> MVKLAEFSRTATFAWSHDKIPLLVSGTVSGTVDANFSTDSSLELWSLLAADSEKPIASLQVDSKFNDLDWSHNNKIIAGALDNGSLELYSTNEANNAINSMARFSNHSSSVKTVKFNAKQDNVLASGGNNGEIFIWDMNKCTESPSNYTPLTPGQSMSSVDEVISLAWNQSLAHVFASAGSSNFASIWDLKAKKEVIHLSYTSPNSGIKQQLSVVEWHPKNSTRVATATGSDNDPSILIWDLRNANTPLQTLNQGHQKGILSLDWCHQDEHLLLSSGRDNTVLLWNPESAEQLSQFPARGNWCFKTKFAPEAPDLFACASFDNKIEVQTLQNLTNTLDEQETETKQQESETDFWNNVSREESKEKPSVFHLQAPTWYGEPSPAAHWAFGGKLVQITPDGKGVSITNPKISGLESNTTLSEALKTKDFKPLINQRLVKVIDDVNEEDWNLLEKLSMDGTEEFLKEALAFDNDESDAQDDANNEKEDDGEEFFQQIETNFQPEGDFSLSGNIEQTISKNLVSGNIKSAVKNSLENDLLMEAMVIALDSNNERLKESVKNAYFAKYGSKSSLSRILYSISKREVDDLVENLDVSQWKFISKAIQNLYPNDIAQRNEMLIKLGDRLKENGHRQDSLTLYLAAGSLDKVASIWLSEFPDLEDKLKKDNKTIYEAHSECLTEFIERFTVFSNFINGSSTINNEQLIAKFLEFINLTTSTGNFELATEFLNSLPSDNEEVKTEKARVLIASGKSLPAQNPATATTSKAKYTNAKTNKNVPVLPTPGMPSTTSIPSMQAPFYGMTPGASANALPPKPYVPATTTSAPVHTEGKYAPPSQPSMASPFVNKTNSSTRLNSFAPPPNPYATATVPATNVSTTSIPQNTFAPIQPGMPIMGDYNAQSSSIPSQPPINAVSGQTPHLNRKANDGWNDLPLKVKEKPSRAKAVSVAPPNILSTPTPLNGIPANAASTMPPPPLSRAPSSVSMVSPPPLHKNSRVPSLVATSESPRASISNPY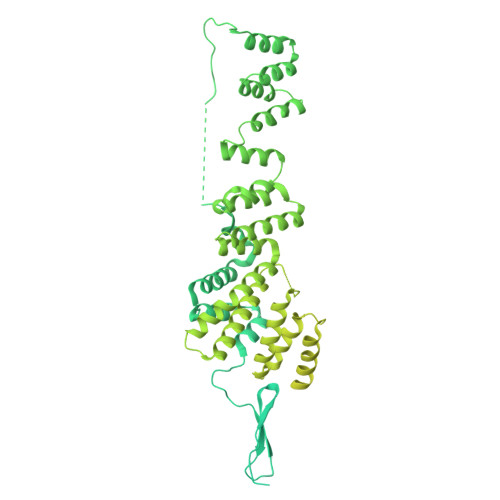APPQSSQQFPIGTISTANQTSNTAQVASSNPYAPPPQQRVATPLSGGVPPAPLPKASNPYAPTATTQPNGSSYPPTGPYTNNHTMTSPPPVFNKPPTGPPPISMKKRSNKLASIEQNPSQGATYPPTLSSSASPLQPSQPPTLASQVNTSAENVSHEIPADQQPIVDFLKEELARVTPLTPKEYSKQLKDCDKRLKILFYHLEKQDLLTQPTIDCLHDLVALMKEKKYKEAMVIHANIATNHAQEGGNWLTGVKRLIGIAEATLN> TAPASTLRFVAVGDWGGVPNAPFHTA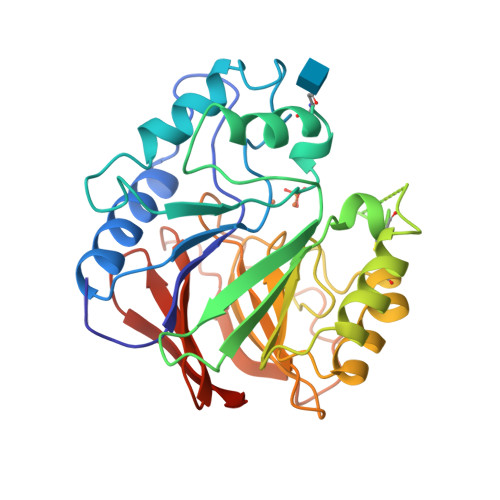REMANAKEIARTVQIMGADFIMSLGDNFYFTGVHDANDKRFQETFEDVFSDRALRNIPWYVLAGNHDHLGNVSAQIAYSKISKRWNFPSPYYRLRFKVPRSNITVAIFMLDTVMLCGNSDDFVSQQPEMPRDLGVARTQLSWLKKQLAAAKEDYVLVAGHYPIWSIAEHGPTRCLVKNLRPLLAAYGVTAYLCGHDHNLQYLQDENGVGYVLSGAGNFMDPSVRHQRKVPNGYLRFHYGSEDSLGGFTYVEIGSKEMSITYVEASGKSLFKTSLPRRPRP>[2x]MGSSHHHHHHSSGMISNRFGQFIDNELADSMISAEKVAHVQLGNNLEHALLVLTKCGYSVIPVLDFEFKLHGLISAAMITDAILGLERIEFERLEDLKVEDVMQTDFPVIKDFNNNERIVHLLVDHPFVCVVDSDHHFEGIVTRRVVLKQVNRYIHLQVEENR

The facultative intracellular pathogen Listeria monocytogenes, like many related Firmicutes, uses the nucleotide second messenger cyclic di-AMP (c-di-AMP) to adapt to changes in nutrient availability, osmotic stress, and the presence of cell wall-acting antibiotics. cbpB encodes a 150-amino-acid protein that is conserved in some Firmicutes. We determined the structures of free CbpB and CbpB in complex with c-di-AMP at 1.6- and 2.4-Å resolution, respectively. These structures reveal that CbpB has tandem CBS domains (CBS1 and CBS2) that interact to form a disk-like head-to-head homodimer. However, here we found that CbpB is a direct activator of RelA and that c-di-AMP inhibits CbpB-dependent RelA activation.

In the c-di-AMP complex, one U-shaped c-di-AMP molecule is bound to each face of the disk, and the binding modes of the two c-di-AMP molecules are essentially the same. One of the adenine bases of c-di-AMP is located in the cleft between the two tandem CBS domains (CBS1 and CBS2) of each monomer, while the other is projected into the solvent. Specific recognition of c-di-AMP is achieved by a large number of hydrogen bonds with both main chains and side chains of CbpB, some of which are mediated by water molecules. The adenine base in the cleft is recognized through hydrogen bonds to its N-1 and N-6 atoms. It is π-stacked against Tyr45 on one face while its other face is flanked by Ile19 and Ile128, thereby forming a narrow pocket for the binding of this base. The 5' phosphate is recognized by hydrogen-bonding interactions with the main chain amide of Arg132, ionic interactions with Arg131 from the other monomer, and hydrogen-bonding interactions with the side chain hydroxyl of Thr130 through a water molecule. In contrast, the other adenine base of c-di-AMP has no hydrogen-bonding interactions with CbpB, and it is not flanked by residues from the protein either, except that its N-6 atom is positioned against Tyr45. Overall, the binding mode of c-di-AMP in CbpB defines a new type of nucleotide recognition by CBS domains.> NIPFTNNLLFSGQVLYGDGRLTAKNHQLVMQGDCNLVLYGGKYGWQSNTHGNGEHCFLRLNHKGELIIKDDDFKTIWSSRSSSKQGEYVLILQDDGFGVIYGPAIFETS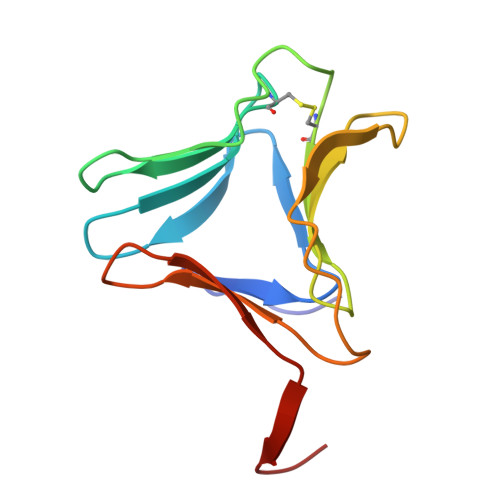S>GMSIVGNVENLINGVGELWNKYVKHEFILKMRDGSLPLDIFRYYLIQDGKYVEDMLRALLIASSKGPIDKVTKILNLVFSSR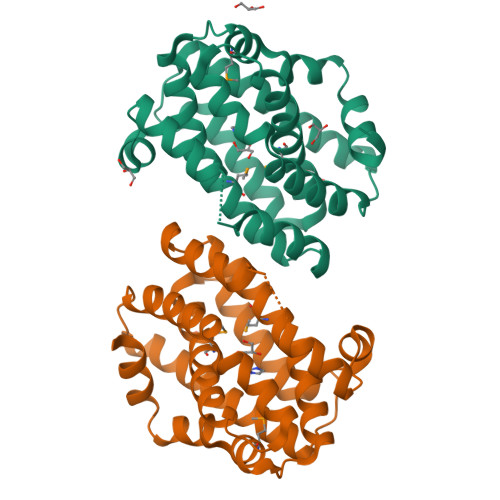DKGLETHGKLYSKLDISRDVIVKTGYNLINYAYTRHLYYYANLDWNKFLVAWTPCMFGYSIVGDYVIDSPNEVYKTWASFYASTEYKKRIEAILYALDEVSITEDLLNIFINSVRFEIGFWDASLRKDPTVY[2x]>[6x]MGQTKSKIKSKYASYLSFIKILLKRGGVKVSTKNLIKLFQIIEQFCPWFPEQGTLDLKDWKRIGKELKQAGRKGNIIPLTVWNDWAIIKAALEPFQTEEDSVSVSDAPGSCIIDCNENTRKKSQKETEGLHCEYVAEPVMAQSTQNVDYNQLQEVIYPETLKLEGKGPELVGPSESKPRGTSPL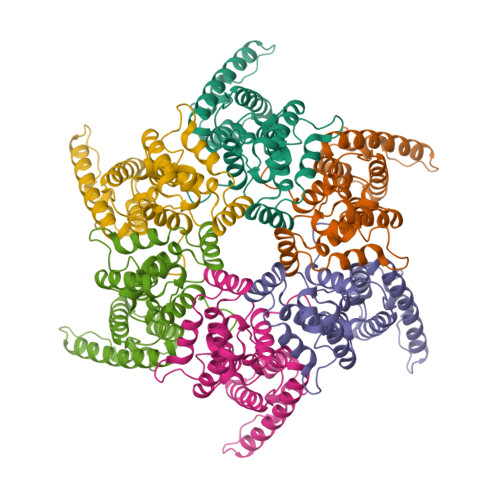PAGQVPVTLQPQKQVKENKTQPPVAYQYWPPAELQYRPPPESQYGYPGMPPAPQGRAPYPQPPTRRLNPTAPPSRQGSELHEIIDKSRKEGDTEAWQFPVTLEPMPPGEGAQEGEPPTVEARYKSFSIKMLKDMKEGVKQYGPNSPYMRTLLDSIAHGHRLIPYDWEILAKSSLSPSQFLQFKTWWIDGVQEQVRRNRAANPPVNIDADQLLGIGQNWSTISQQALMQNEAIEQVRAICLRAWEKIQDPGSTCPSFNTVRQGSKEPYPDFVARLQDVAQKSIADEKARKVIVELMAYENANPECQSAIKPLKGKVPAGSDVISEYVKACDGIGGAMHKAMLMAQAITGVVLGGQVRTFGGKCYNCGQIGHLKKNCPVLNKQNITIQATTTGREPPDLCPRCKKGKHWASQCRSKFDKNGQPLSGNEQRGQPQAPQQTGAFPIQPFVPQGFQGQQPPLSQVFQGISQLPQYNNCPPPQAAVQQ>[3x]MDIPRIFTISESEHRIHNPFTEEKYATLGRVLRMKPGTRILDLGSGSGEMLCTWARDHGITGTGIDMSSLFTAQAKRRAEELGVSERVHFIHNDAAGYVANEKCDVAACVGATWIAGGFAGAEELLAQSLKPGGIMLIGEPYWRQLPATEEIAQACGVSSTSDFLTLPGLVGAFDDLGYDVVEMVLADQEGWDRYEAAKWLTMRRWLE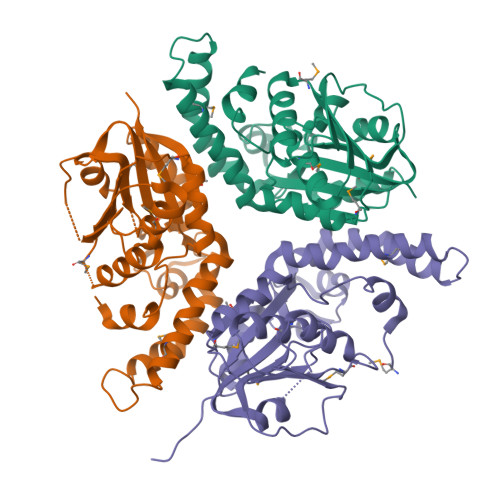ANPDDDFAAEVRAELNIAPKRYVTYARECFGWGVFALIARLEHHHHHH YceI proteins are a family of bacterial lipocalins (BCNs), which are small proteins widely conserved in Gram-negative and Gram-positive bacteria but whose physiological role is unclear. In this study, we discovered that secreted BCNs contribute to antibiotic resistance by capturing and neutralizing antibiotics in the bacterial milieu. Visual inspection and structural alignments by the DALI server confirmed a barrel-shaped lipocalin fold for both proteins. An octaprenyl pyrophosphate was bound within a long, hydrophobic tunnel extending from one end of the barrel in each structure.

To elucidate the mode of binding of antibiotics within BCNs, we first solved the X-ray crystal structures of BcnA and BcnB to 1.4- and 1.6-Å resolutions, respectively. Analysis with the PDBePISA server predicted that BcnA is a monomer, while BcnB is a dimer, by crystallographic symmetry (~2,840 Å2 of buried surface area including a portion of the tunnel opening). These oligomeric states were confirmed in solution by size exclusion chromatography-multiangle light scattering (SEC-MALS). Superposition of BcnA chain A and BcnB chain C (148 Cα atoms, 22% sequence identity) resulted in a root mean square deviation (RMSD) of 1.66 Å. The largest structural differences observed were located in two of the loops that make up the tunnel opening. These differences may play a role in the antibiotic binding potential of BcnA and BcnB. Notably, the binding of BcnB to Nile red occurred with ~20-fold lower affinity than that of BcnA, agreeing with the lesser role of BcnB in antibiotic resistance. The secretion of the BcnA and BcnB proteins was also investigated by using FLAG-tagged derivatives; only BcnA was secreted extracellularly into the growth medium. The ΔbcnA mutant, but not the ΔbcnB mutant, had increased susceptibility (4-fold MIC reduction) to rifampin, norfloxacin, ceftazidime, and the cationic antimicrobial peptide polymyxin B (PmB) and a 2-fold meropenem MIC reduction.

>SATYQFDPSHTYPSFEADHFGGLSVWRGKFDKSSGTVTLDRAAKTGTVDVTTDIASIHTGSAKLDEHLQTAEFFDAAKFPQANYKGTIKFDGDKPVSVVGNLTLHGVTKPLTLKIDSFKCMPHPMLKREVCGVDAVGEFSRDDFGLDYGKQYGFKMKTKLLITAEAVKQ[4x]>MAHHHHHHVREEKLRLRKQII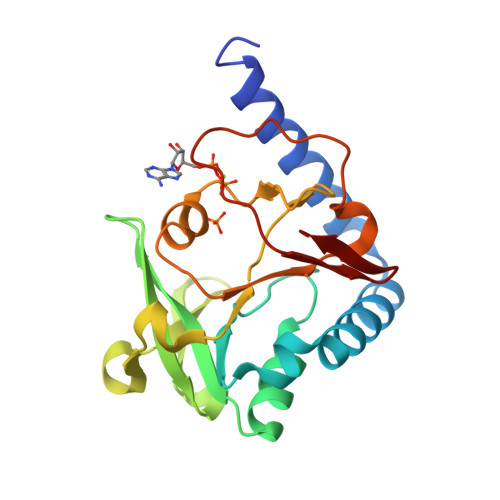EHMNSLSKERYTTLSEQIVFSLYEQKEWAEAKTIGITLSMENEVNTYPIIEKAWKEGKRVVVPKCNKETRTMSFRQISNFDQLETVYMNLREPIPALTEEVNADEIDLQIVPGVAYTERGERIGYGGGYYDRYLVHYKGKTLSLAYSFQMVEHIPVEPFDKNVEKIITEKGTMVKNGLV[2x]ethyl 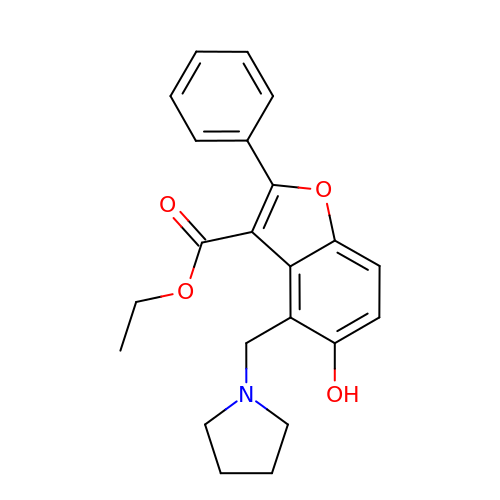5-hydroxy-2-phenyl-4-(pyrrolidin-1-ylmethyl)-1-benzofuran-3-carboxylate | C22 H23 N O4 | VIMMVCAKDVTEMS-UHFFFAOYSA-N>[2x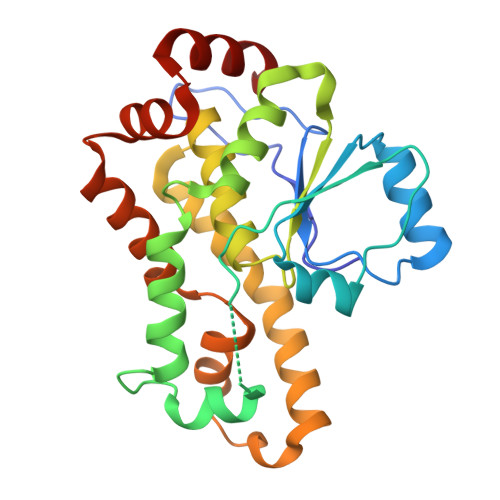]GGGMKNFRDLGGNKTEDGRTVKKGLFYRSAKLSNLSENDIKILKELNIKYIFDYRSDEEARKHPSTIISNIKNIRIPAMRELEESGGSFGSIEDMIDGLFEKDGAFNMLNNSYYNLPINNPSYKKLVELIRDYSNLPILNHCTAGKDRTGVGSAIILMILGVSRENIMKDYLKSNDFADKEIERFIEYKPKFKDIPKENLKYIFGVNEEYMKTAFRRIDEEYISVEAYLYGEFNLNKEEIRKLRNQYLE>[2x]NECLGTIGPVTPLDASDFALDIRMPGVTPKESDTYFCMSMRLPVDEEAFVIDFKPRASMDTVAHMLLFGCNMPSSTGSYWFCDEGTCTDKANILYAWARNAPPTRLPKGVGFRVGGETGSKYFVLQVHYGDISAFRDNHKDCSGVSVHLTRVPQPLIAGMYLMMSVDTVIPPGEKVVNADISCQYKMYPMHV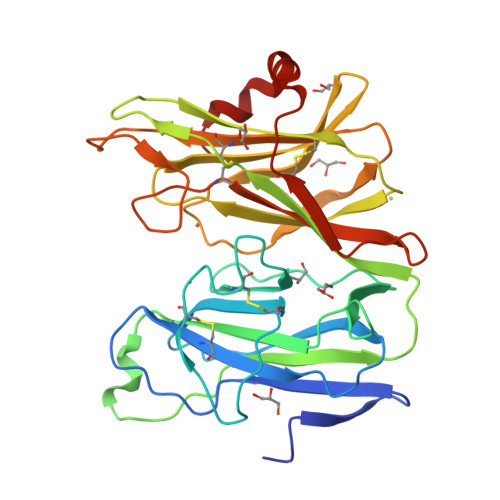FAYRVHTHHLGKVVSGYRVRNGQWTLIGRQNPQLPQAFYPVEHPVDVTFGDILAARCVFTGEGRTEATHIGGTSSDEMCNLYIMYYMEAKYALSFMTCTKNVAPDMFRTIPAEANIPIPV>AYSNTYQEFTNIDQAKAWGNAQYKKYGLSKSEKEAIVSYTKSASEINGKLRQNKGVINGFPSNLIKQVELLDKSFNKMKTPENIMLFRGDDPAYLGTEFQNTLLNSNGTINKTAFEKAKAKFLNKDRLEYGYISTSLMNVSQFAGRPIITKFKVAKGSKAGYIDPISAFAGQLNMLLPRHSTYHIDDMRLSSDGKQIIITATMMGTA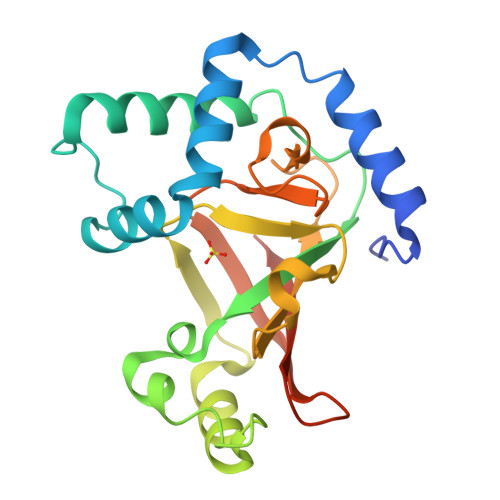INPK[3x]>[3x]MHHHHHHSSGLVPRGSMI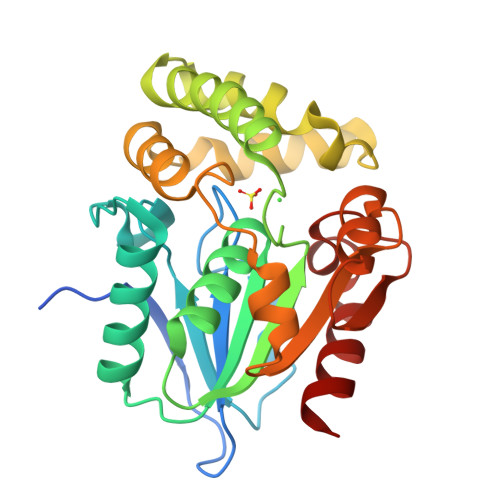LHAQAKHGKPGLPWLVFLHGFSGDCHEWQEVGEAFADYSRLYVDLPGHGGSAAISVDGFDDVTDLLRKTLVSYNILDFWLVGYSLGGRVAMMAACQGLAGLCGVIVEGGHPGLQNAEQRAERQRSDRQWVQRFLTEPLTAVFADWYQQPVFASLNDDQRRELVALRSNNNGATLAAMLEATSLAVQPDLRANLSARTFAFYYLCGERDSKFRALAAELAADCHVIPRAGHNAHRENPAGVIASLAQILRF>MSGSHHHHHHSGSMSERPSDLVVNRLVLFVVKGTATSTHNTVKPLILLEELGVPHDIYVVEKVSAPWFSEINPHKMVPAILDRSPDGRDTLRA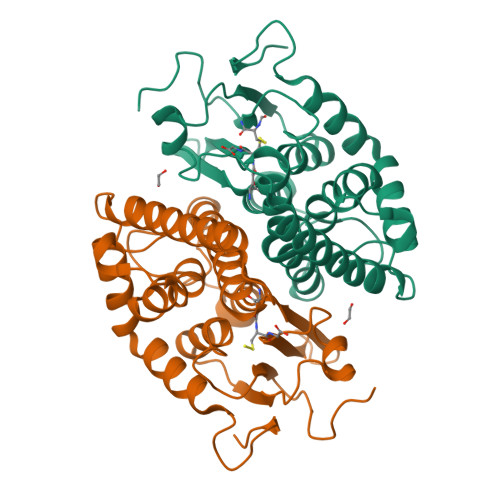WESTSTLMYIADAYDKDGTFGGRNVQERSEINNWLTLHTAALGPTAGYWLYFYKLHPEKLPKTIEKLRSNITVQYDILERRLNEPGQQYLALKDRPTIADIATLPFAMKSTAELFGLEFEKWPKLQEWSVRMGEREAVKRAWQRVAGFGHGEKEYGMLEA[2x]>[8x]HHHHHHLEVLFQGPMKYTKLEKDALDLLSDNEEEDAESSILTFEERDTSSLSIEARLESIEEKLSMILGLLRTLNIATAGPTAARDGIRDAMIGVREELIADIIKEAKGKAAEMMEEE

The essential polymerase cofactor P from Pneumoviridae is a multifunctional hub which interacts with numerous components of the viral RNA-synthesis machinery. Pneumoviral P interacts with both L and the nucleocapsid, thereby tethering the polymerase to its template. In HMPV and RSV a central oligomerization domain facilitates the formation of P tetramers. In summary, we have shown that HMPV P is a highly dynamic protein that is composed of a stable helical tetramerization domain flanked by large N-terminal and C-terminal IDRs that sample a large volume in solution and display varying degrees of preformed structural elements.

Although we were not able to grow crystals of a complex, crystals which later proved to harbour only the P oligomerization region could be obtained after extended time periods. Serendipitously, we obtained two additional crystal forms of Pcore with improved resolution, allowing us to build a higher quality model (100% Ramachandran favoured). The first crystal (form 1, space group P21) diffracted to a resolution of 1.6 Å, while the second crystal (form 2, space group P212121) gave rise to diffraction data up to 2.2 Å. The P212121 crystal (form 2) grew at 20 °C after between 132 and 185 days with mother liquor containing 25% PEG 3350, 200 mM MgCl, and 100 mM Tris, pH 8.5. Diffraction data were recorded on beamlines I03 (P21 crystal) and I04 (P212121 crystal) at Diamond Light Source, Didcot, UK. In one of the tetramers within crystal form 2 we observed a single, solvent-exposed helix which possessed markedly blurred electron density and, as a result, significantly higher crystallographic B-factors than the three other protomers of the coiled-coil (white arrow). This suggests that, in absence of packing constraints within the crystal (as is the case for this solvent-exposed helix), the protomers of the Pcore region are somewhat flexible and there is a certain degree of malleability of the tetramer interface. Alignment of all six tetramers from crystal forms 1 and 2 and the original crystal confirmed that there are small-scale breathing motions within the coiled-coil. This is fully consistent with the overall lower buried surface area (~4800 Å) and predicted dissociation energy (~21 kcal/mol) for HMPV P than in the more extended paramyxoviral coiled-coil oligomerization domains. For comparison, the buried surface area and predicted dissociation energy of the Nipah virus P oligomerization domain have been reported to lie between 15000–20000 Å and 140–200 kcal/mol. These data indicate a flexibly associated tetramer of HMPV P protomers.2-chloro-2'-deoxyadenosine | C10 H12 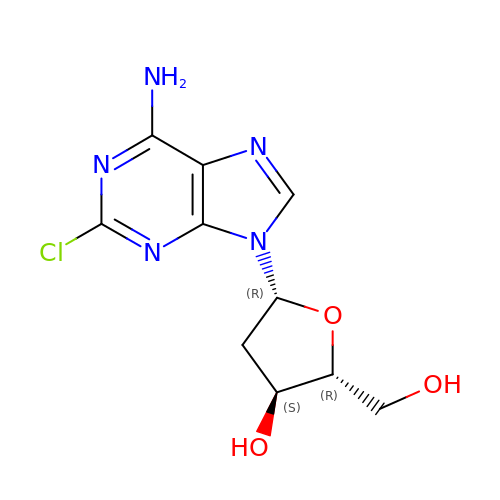Cl N5 O3 | PTOAARAWEBMLNO-KVQBGUIXSA-N> MAADAPGDRMEEPLPDRAVPIYVAGFLALYDS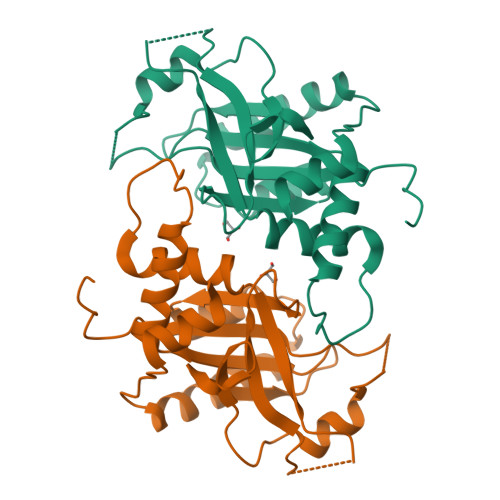GDSGELALDPDTVRAALPPDNPLPINVDHRAGCEVGRVLAVVDDPRGPFFVGLIACVQLERVLETAASAAIFERRGPPLSREERLLYLITNYLPSVSLATKRLGGEAHPDRTLFAHVALCAIGRRLGTIVTYDTGLDAAIAPFRHLSPASREGARRLAAEAELALSGRTWAPGVEALTHTLLSTAVNNMMLRDRWSLVAERRRQAGIAGHTYLQA> SSGIHVALVTGGNKGIGLAIVRDLCRLFSGDVVLTARDVTRGQAAVQQLQAEGLSPRFHQLDIDDLQSIRALRDFLRKEYGGLDVLVNNAGIAFKVADPTPFHIQAEVTMKTNFFGTRDVCTELLPLIKPQGRVVNVSSIMSVRALKSCSPELQQKFRSETITEEELVGLMNKFVEDTKKGVHQKEGWPSSAYGVTKIGVTVLSRIHARKLSEQRKGDKILLNACCPGWVRTDMAGPKATKSPEEGAETPVYLALLPPDAEGPHGQFVSEKRVEQW

The carbonyl reductase CBR1 was first isolated from brain and has been associated with two cellular functions: (1) detoxification of xenobiotics, such as the anthracycline daunorubicin and (2) metabolism of ketone-containing cellular messengers, such as prostaglandin E. Genetic studies that have intended to uncover the in vivo function of this enzyme have focused on the xenobiotic detoxification activity of the enzyme. Using matrix-assisted laser desorption/ionization (MALDI) and electrospray ionization (ESI) MS/MS sequencing, B1–B3 were each identified as human CBR1, a member of the short-chain dehydrogenase/reductase family of NAD(P)(H) oxidoreductases. CBR1 converts daunorubicin into daunorubicinol, a compound that lacks the anti-proliferative activity of the parent daunorubicin and is cardiotoxic. We used affinity purification to identify a target of hydroxy-PP, carbonyl reductase 1 (CBR1), a short-chain dehydrogenase-reductase.

We overexpressed human CBR1 in Escherichia coli and attempted crystallization of the protein in the presence of hydroxy-PP in an effort to enhance design of a selective CBR1 inhibitor. The structure was solved by molecular replacement with the AMoRe program using a modified porcine carbonyl reductase model and refined with SHELXL to 1.24 Å with a crystallographic R-factor of 10.3% and a free R-factor of 13.4%. Although NADP(H) was not present during purification of the enzyme from E. coli nor added to the crystallization experiments, one molecule of NADP was found to be bound in the CBR1–hydroxy-PP structure. Hydroxy-PP binds to the substrate-binding site of CBR1, with the pyrazolopyrimidine core of hydroxy-PP mainly surrounded by hydrophobic residues (Trp229, Met141, and Ile140). The phenolic hydroxyl group of hydroxy-PP, however, points deep into the substrate-binding pocket and interacts with Tyr139 and Ser193 of the catalytic triad. The phenolic oxygen is positioned 2.5 Å from Oη of Tyr139 and 2.5 Å from Oγ of Ser193, thus indicating strong hydrogen bonding. The C4 carbon of the NADP(H) nicotinamide ring is positioned 3.2 Å from the meta-hydroxy carbon. Importantly, the structure of CBR1–hydroxy-PP provides a molecular understanding of the basis for the strong dependence of CBR1 inhibition on the presence of a hydroxyl moiety, as this functional group serves as a key interaction determinant with the catalytic machinery of CBR1. The binding mode of hydroxy-PP in CBR1 also explains the tolerance of the pyrazolopyrimidine core to derivatization at N-1, which allowed attachment of hydroxy-PP to solid support and affinity purification of CBR1. Importantly, structural analysis of the hydroxy-PP–CBR1 co-crystal structure revealed a small space in the active site capable of tolerating a methyl substituent at this position.> GSPELRQEHQQLAQEFQQLLQEIQQLGR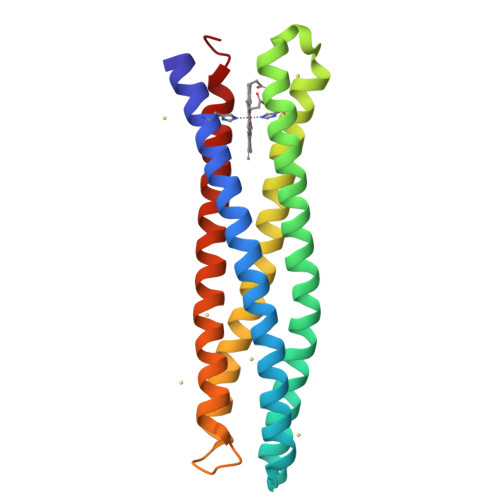ELLKGELQGIKQLREASEKARNPEKKSVLQKILEDEEKHIELHETLQQTGQEAQQLLQELQQTGQELWQLGGSGGPELRQKHQQLAQKIQQLLQKHQQLGAKILEDEEKHIELLETILGGSGGDELRELLKGELQGIKQYRELQQLGQKAQQLVQKLQQTGQKLWQLG>[2x]SMIGLTAGEPAYLHPLLHQNTSTLSEQRYSSTFTGQEFFLRDHVVNGQKVLPGVAYLEMARVAVDMAAGVRTDNHSAIQLKNIVWAKPVIVEDAPIQVHKGLYPEENGEITFEIYSHPREAEESLVVHSQGRAVLRSAMEAPALDLSAIQAQ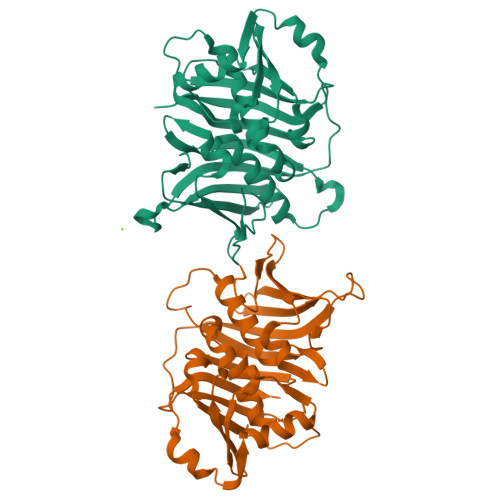CTESSYSFSQCYETFHRIGLAYGPSHQGIEKLFVGPDQVLAKLVLPSSVTGTAEKFVLHPSVMDAALQASLGFMMGTSDLQPSLPFALEELNIYSASTAAAWALVRYSDGNATTQKVQKLDIDLCDEQGTICVSMKGFTTRVLEGEKAAGVAKNKGTGEAGKITSTLMLQPVWIEKGIPKEAKA> MSLYHKILIGFVLGVIVGLIFGDKAEFIKPLGDIFLRLLKMIVVPLVFSTIVTGIASMGDVKKLGRIGAKTLIYYMITTTLAV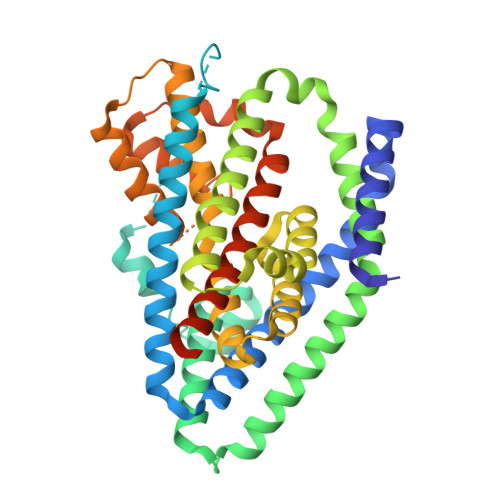TIGLILANIFKPGKGLSLGEIHEVAHPNAPSFTETLLNMIPTNPFEAMAEGNMLQIIVFAIFFGIALALMGEKAEPVKKFFDSASEVMFKITDIVMKFAPYGVFALMAWTVGKYGLDVLAPLGKLILTVYLGCIIHILIVYTLLLRFLCKINPLRFFKKIKEAMLVAFSTCSSAATLPVTMRVAEELGVPESIASFTLPLGATINMDGTALYQGVAAIFVAQAYGVELTLGQQLTIVLTAVLASIGTAGVPGAGLVMLTMVLTSVGLPLEGIALIAGIDRILDMARTTVNVTGDLVATAIVARTENELNREMTATPLEVLESKTIAL> GSGMMRYLHKIELELNRLTSRYPFFKKIAFDAEIIKLVDDLNVDENVKCAIVAIDTSMRMQDFINEDNKDSFVLSTDVLSALFYKYLSQPFYQHDFLVLTDCV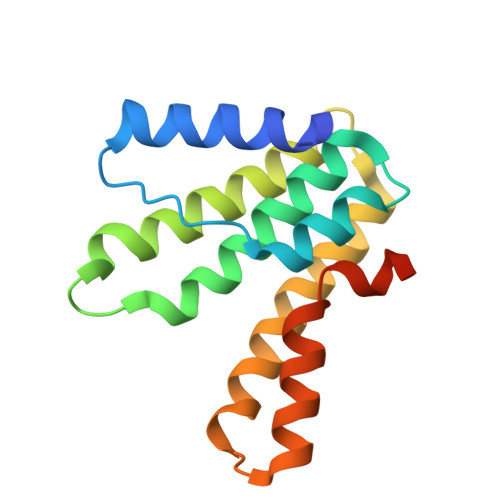SRINELKSIRATITDEIALHNINKQIHYMFIQPYMNNEKVVSYE>MLAKDKVALLIGNMNYREHPKLKAPLVDVYELTNLLRQLDFKVVSLLDLTEYEMRNAVDEFLLLLDKGVYGLLYYAGHGYENFGNSFMVPVDAPNPYRSENCLCVQNILKLMQEKETGLNVFLLDMCRKRNDYDDTIPILDALKVTANIVFGYATCQGAEAFEIQHSGLANGIFMKFLKDRLLEDKKITVLLDEVAEDMGKCHLTKGKQALEIRSSLSEKRALTDPIQGTEYSAESLVRNLQWAKAHELPESMCLKFKCGVQIQLGFAAEFSNVMIIYTKIVYKPPEIIMCDAYVTDFPLDLDID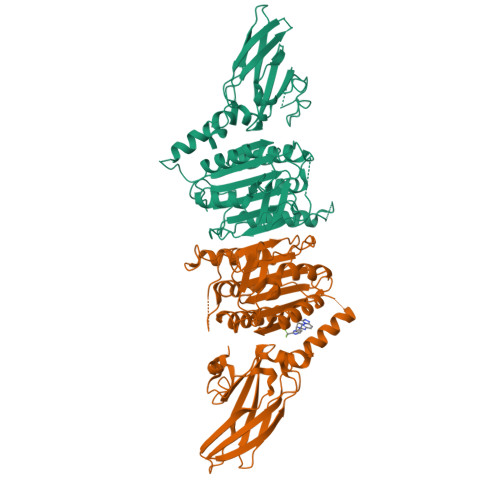PKDANKGTPEETGSYLVSKDLPKACLYTRLSSLQKLKEELVFTVCLSYQYSGLEDTVEDKQEVNVGKPLIAKLDMHRHHHHHH[2x]>MHHHHHHHHENLYFQGSDGDVKPAKPAVVLEA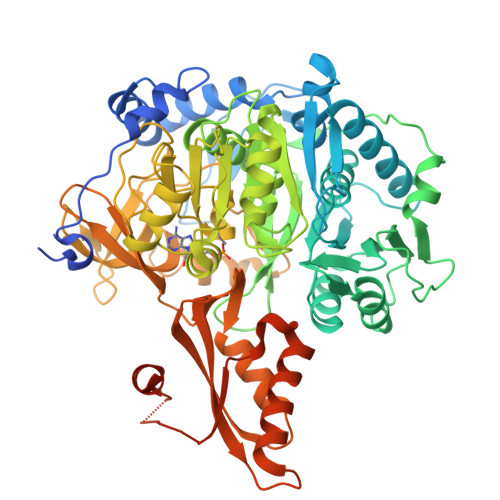NDVDTFHVPKAFYEKHPSKTHLKDLDEYKKLYDESIRSPDTFWARMARELLTFDKDFQTTHIGSLENGDNAWFVEGRLNASFNCVDRHAIKNPNKVAIIYEADEPNEGRIITYGELLREVSRVAWVLKQRGVKKGDTVAIYLPMIPEAVVAFLACARIGAIHSVVFAGFSSDSLRDRVLDAGSKVVITTDEGKRGGKVIGTKRIVDEALKQCPDVTSVLVYKRTGAEVPWTNGRDIWWHEEVEKYPCYVAPESMSSEDPLFLLYTSGSTGKPKGVMHTTAGYLLGAAMTGKYVFDIHDDDRFFCGGDVGWITGHTYVVYAPLLLGCSTVVFESTPAYPNFSRYWDVIEKHKVTQFYVAPTALRLLKRAGDEHIHHKMEHLRILGSVGEPIAAEVWKWYFEKVGKEEAHICDTYWQTETGSHVISPLGGITSTKPGSASLPFFGIEPAIIDPVSGEEISGNDVEGVLAFKQPWPSMARTVWGAHKRYMDTYLNVYKGYYFTGDGAGRDHDGYYWIRGRVDDVVNVSGHRLSTAEIEAALIEHHQVAEAAVVGIADELTGQAVNAFVSLKDGNETTEQVRKDLVMQVRKSIGPFAAPKAVFVVEDLPKTRSGKIMRRILRKILSGEEDSLGDTSTLSDPSVVNKIIETVHAARAK[6x]> DAMDITVSIPPQQYFLEKIGGDLVRVSVLVPGNNDPHTYEPKPQQ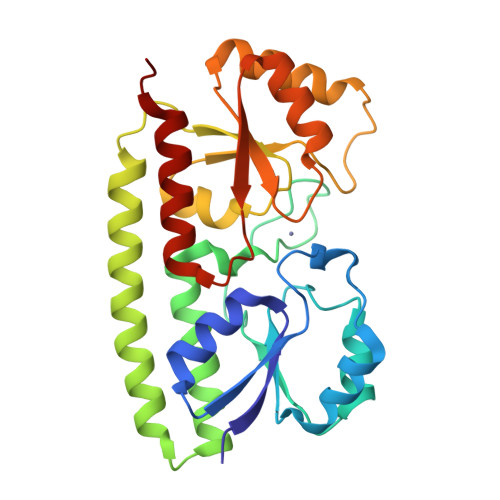LAALSEAEAYVLIGLGFEQPWLEKLKAANANMKLIDSAQGITPLEMPGRLMVADPHIWLSPTLVKRQATTIAKELAELDPDNRDQYEANLAAFLAELERLNQELGQILQPLPQRKFIVFHPSWAYFARDYNLVQIPIEVEGQEPSAQELKQLIDTAKENNLTMVFGETQFSTKSSEAIAAEIGAGVELLDPLAADWSSNLKAVAQKIANANSAQP> MPIIKEPIDFINKPESEAKEWGKEEEKRWFTKLNNLEEVAVNQLKNKEYKTKIDNFSTDILFSSLTAIEIMKEDENQNLFDVERIREALLKNTLDRDAIGYVNFTPKELGINFSIRDVELDRDISDETLDKVRQQIINQEYTKFSFISLGLNDNSINESVPVIVKTRVPTTFDYGVLNDKETVSLLLNQGFSIIPESAIITTIKGKDYILIEGSLSQELDFYNKGSEAWGAENYGDYISKLSHEQLGALEGYLHSDYKAINSYLRNNRVPNNDELNKKIELISSALSVKPIPQTLIAYRRVDGIPFDLPSDFSFDKKENGEIIADKQKLNEFIDKW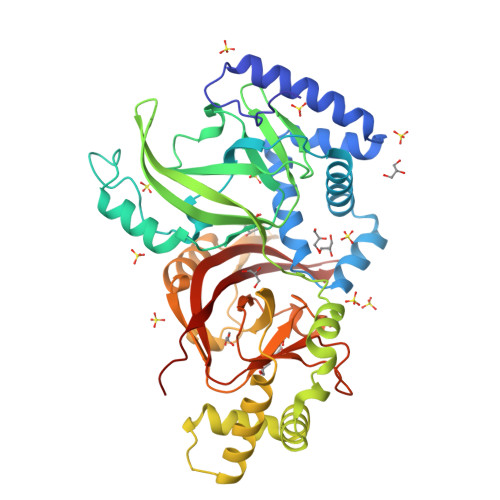TGKEIENLSFSSTSLKSTPSSFSKRRFIFRLRLSEGAIGAFIYGFSGFQDEQEILLNKNSTFKIFRITPITSIINRVTKMTQVVIDAEGIQNKEI>[2x]MKYRCKVCDYIYDPEVGDPTSGIKPGTPFQELPEDWLCPV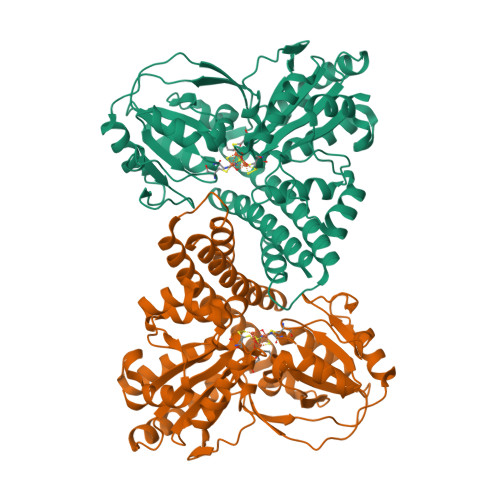CNVGKDQFEPLRGEVRRVRPEDIDMFYYQCSQTVRGRACTVKGVCGKEATVARLQDNLLFAIKGISAYLYHARELGYTDEVVDAFLERGFYSTLTNVNFDAEEFVSLALEAGEMNLRTMKLLKKAHMDTYGEPEPAEVRVGALDGPAIIATGHSLKALEELLKQTEGSGVNVYTHSELLPAHGYPGLRKYPHLAGQLGGPWFDQRETFSRYSAAVLGTSNCVLLPRDSYRDRMFTCGVARLPGVEHVDGYDFSPVIEKALELPPLKEEDSATLTTGFGLSTILSLADKIKELVEEGKIRRFFLVGGCDSPLPQAKYYTEFVRKLPEDTVVLTLACGKYRFNSMDLGDIDGIPRLIDLGQCNDSIVAVELVEALSNLFSMDVNELPLSIVLSWMEQKAAAILWSLLSLNLRGMYIGPILPGWANDDIINVLVDKYELTPIGDPEEDIKKMMEVDKLAAALEHHHHHH>[8x]MTQSVSLSDFIVKTEDGYMPSDRECVALDRYLSKEQKELRETFKDGKNDRSALRIKMFLSPSPSRRFTQHGVVPMREIKTNTDIPSTLWTLVTDWLLNLLQDEENQEMFEDFISSKFPDVLASADKLARFAQRLEDRKDVLHKNFSKAMNAFGACFWAIKPTFATEGKCNVVRATDDSMILEFQPVPEYFRCGRSKATFYKLYPLSDEQPVNGMLALKAVAGNQFFMYHGHGHIRTVPYH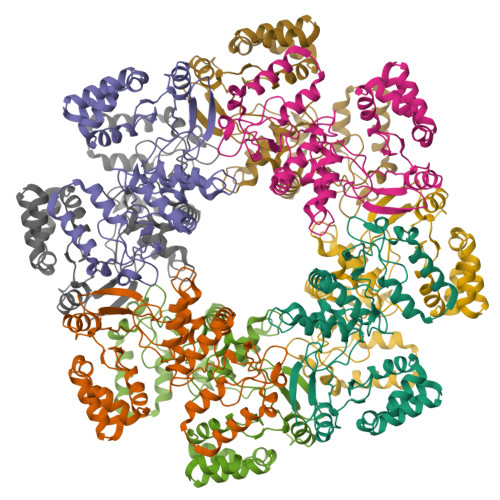ELADAIKSYARKDKETLESISKSPLAAQCGSKFLDMLDGIRSKQKIEDVILKAKIFEKKRS> TALTLVEQILAEFQLQEEDLKKVMRRMQKEMDRGLRLETHEEASVKMLPTYVRSTPEGSEVGDFLSLDLGGTNFRVMLVKVGEGEEGQWSVKTKHQMYSIPEDAMTGTAEMLFDYISECISDFLDKHQMKHKKLPLGFTFSFPVRHEDIDKGILLNWTKGFKASG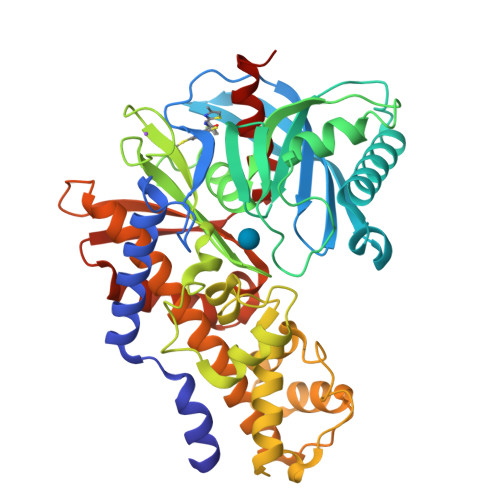AEGNNVVGLLRDAIKRRGDFEMDVVAMVNDTVATMISCYYEDHQCEVGMIVGTGCNACYMEEMQNVELVEGDEGRMCVNTEWGAFGDSGELDEFLLEYDRLVDESSANPGQQLYEKLIGGKYMGELVRLVLLRLVDENLLFHGEASEQLRTRGAFETRFVSQVESDTGDRKQIYNILSTLGLRPSTTDCDIVRRACESVSTRAAHMCSAGLAGVINRMRESRSEDVMRITVGVDGSVYKLHPSFKERFHASVRRLTPSCEITFIESEEGSGRGAALVSAVACKKACMLGQ>[6x]MGSDKIHHHHHHMKVYFDDIYVSTARQFELVDITDQVEQIVEKSGIKNGICLIFVAHSTAAIVANEHER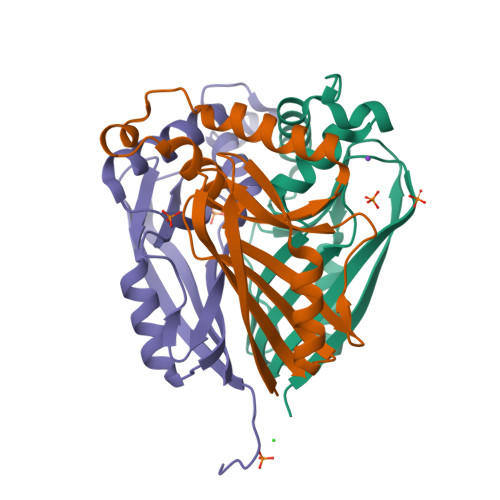GLMEDILTKIKEFTEPSRSWKHNLIDDNAHAHLGATFLGAERVFPVREGKLVRGTWQNIFLVELDGPRSERHITVEILGE>MTNIDVRWQQRLNNYARALQQLSLAVNLAQTRPLSDLEKQGLIQAFEFTHELAWNVMKDYFFFQGNSAITGSRDATRESFNKGLIKEGEIWMEMIKSRNQTSHTYNQSVADEIVKNIINFYHTSFQAFLEKMQGLKEHE[4x];>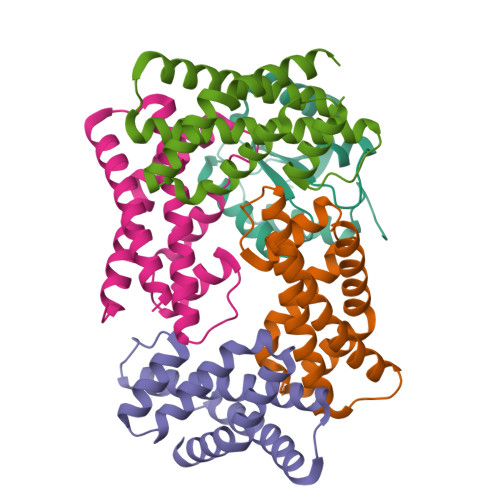 MNEQLNHLYGLPSHAIEALKCVFKEYSQIDNAILYGSRAKGTYHQGSDIDLCLTGNLLGITELLAIENKIDDLLLPWKVDISLKHTIDNPDLLEHIERAGILFYTKES A new family of protein tyrosine-kinases harboring a P-loop type nucleotide binding-domain with a Walker A motif has been described. They have been called BY-kinases (Bacterial-tyrosine-kinases) as they are only found in bacterial genomes. BY-kinase autophosphorylation on a C-terminal tyrosine cluster, called Y-cluster is crucial in regulating polysaccharide export. In firmicutes, the situation is quite similar except that BY-kinases are split into two proteins: one corresponds to the cytoplasmic catalytic domain of proteobacterial BY-kinases (about 230 residues) and the other is a transmembrane domain homologous to the Wzz-like domain (about 230 residues) of proteobacterial BY-kinases.

In order to find out the structural basis of this discrepancy, we solved the crystal structure of the chimera CapA2B2 (last 27 C-terminal amino acids of CapA2 fused to the N-terminus of CapB2). Previous mass spectrometry analysis demonstrated indeed that each band corresponds to a different phosphorylation level, from 0 to 4 phosphorylated residues among the 4 tyrosines 221, 222, 224 and 225 of the Y-cluster. This result demonstrated that the Y-cluster of the CapA2B2 chimera from S. aureus autophosphorylated spontaneously during its production process in E. coli cells. Autophosphorylation was however less efficient than for CapA1B2 since addition of ATP was required to observe the fully phosphorylated form of CapA2B2. As previously observed in the CapA1B2/ADP-Mg complex, the phosphorylated C-terminal Y-cluster of CapB2 is disordered and analysis of the crystal contacts using PISA confirmed that the protein is a monomer. The CapA2 N-terminal part of the protein adopts the same αA-βA conformation than that of the CapA1 fragment. Interestingly, CapB2 residues 1 to 8 linking βA to helix α1 are disordered. Unlike the CapA1B2(K55M) structure that contained bound ADP-Mg while no nucleotide was added to the crystallization solution, the active site of CapA2B2 did not reveal any electron density corresponding to a nucleotide that would have co-purified from E. coli. This is in agreement with a previous study showing that CapA2B2 displays a weaker affinity for nucleotides compared to CapA1B2, with respective Kd values for Mant-ATP of 190 nM and 50 nM. In the apo structure of CapA2B2, Phe220 is slightly shifted compared to the CapA1 Phe221 residue stacked against the bound adenine in the CapA1B2/ADP-Mg complex. The reduced activation efficiency of CapA2 could be explained by the absence of the CapA1 last residue Asn222 that interacts with the N-terminus of CapB2.

> MRGSHHHHHHGSLLDKRIKTEEDVESQLGLPILGSIQKFMTNTRRSTSSLIVHEQPKSPISEKFRGIRSNIMFANPDSAVQSIVITSEAPGAGKSTIAANLAVAYAQAGYKTLIVDGDMRKPTQHYIFNLPNNEGLSSLLLNWSTYQDSIISTEIEDLDVLTSGPIPPNPSELITSRAFANLYDTLLMNYNFVIIDTPPVNTVTDAQLFSKFTGNVVYVVNSENNNKDEVKKGKELIEATGAKLLGVVLNRMPKDKSASYYAYYGTDES>[3x]MASLRSRCDQLEERVSAAEDEINEIKREGKFREKRIKR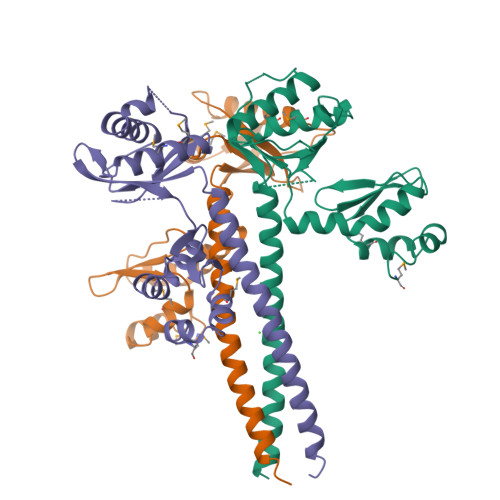NEQSLQEIWDYVKRPNLRLIGVPESDVENGTKLENTLQDIIQENFPNLARQANVQIQEIQRTPQRYSSRRATPRHIIVRFTKVEMKEKMLRAAREKGRVTLKGKPIRLTVDLSAETLQARREWGPIFNILKEKNFQPRISYPAKLSFISEGEIKYFIDKQMLRDFVTTRPALKELLKEALNMERNHHHHHH>MGSSHHHHHHENLYFQSMASMKTELIRTISLYDTIILHRHVRPDPDAYGSQCGLTEILRETYPEKNIFAVGTPEPSLSFLYSLDEVDNETYEGALVIVCDTANQERIDDQRYPSGAKLMKIDHHPNEDPYGDLLWVDTSASSVSEMIYELYLEGKEHGWKLNTKAAELIYAGIVGDTGRFLFPNTTEKTLKYAGELIQYPFSSSELFNQLYETKLNVVKLNGFIFQNVSLSENGAASVFIKKDTLEKFGTTASEASQLVGTLGNISGIRAWVFFVEEDDQIRVRFRSKGPVINGLARKYNGGGHPLASGASIYSWDEADRILADLETLCKEHE[4x]

In the Firmicute B. subtilis, the ytqI gene product was shown to be a major nanoRNA turnover enzyme, and was renamed NanoRNase A (NrnA). We show here that Bacillus NrnA is a bidirectional nuclease that can degrade RNA fragments from either the 3′ or the 5′ end. We have determined crystal structures of B. subtilis NrnA in its apo form, as well as complexed with substrates. These structures reveal a dynamic bi-lobed molecule with the DHH catalytic domain and the DHHA1 substrate binding domains connected through an extended linker.

Bacillus NrnA was crystallized in the P21 space group with four molecules per asymmetric unit. The B. subtilis NrnA structure comprises two globular domains connected by a linker region (residues 178–194) that consists of a short α-helix bordered by two loops. The N-terminal DHH catalytic domain adopts a mixed α/β fold featuring a 5-stranded parallel β-sheet at its core. Residues from the DHH motifs come together to form a surface-exposed active site that faces the C-terminal substrate-binding domain. The C-terminal DHHA1 domain of NrnA also adopts an α/β fold with a central mixed β-sheet and helices on both the apical and basal sides. The four NrnA molecules in the P21 asymmetric unit of our crystal structures display variation in the orientation of the C-terminal DHHA1 domain with respect to the DHH domain, and the distances between Cα of H284 (at the end of the GGGH motif) and Cα of H104 (in the DHH active site) can vary from 11.9 to 19.3 Å. NrnA from B. fragilis, M. smegmatis and M. tuberculosis are reported to be dimeric, and Bacillis NrnA in our crystals packs in a similar manner. The dimer interface in Bacillus NrnA covers about 1600 Å2, 11% of the total surface area of the molecule, and is centered around helices α5 and α9. Whether dimerization is a consequence of crystal packing or is the physiologically active entity is unclear. In either case, the NrnA active site directly faces the DHHA1 domain of the same monomer and away from the dimerization interface, indicating the catalytic cycle of an individual nanoRNA occurs within one monomer.>[5x]GMEVLDLVTGPDSVTEIEAFLNPRMGQPPTPESLTEGGQYYGWSRGINLATSDTEDSPENNTLPTWSMAKLQLPMLNEDLTCDTLQMWEAVSVKTEVVGSGSLLDVHGFNKPTDTVNTKGISTPVEGSQYHVFAVGGEPLDLQGLVTDARTKYKEEGVVTIKTITKKDMVNKDQVLNPISKAKLDKDGMYPVEIWHPDPAKNENTRYFGNYTGGTTTPPVLQFTNTLTTV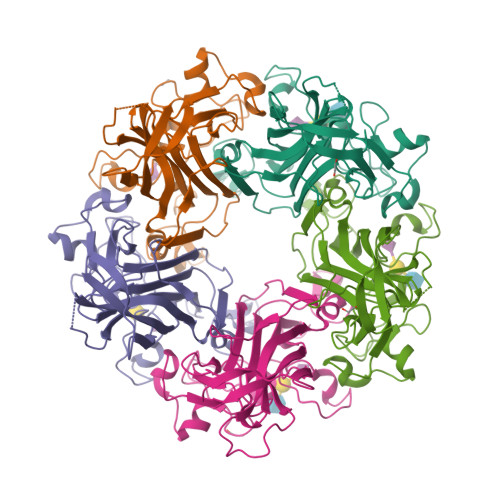LLDENGVGPLCKGEGLYLSCVDIMGWRVTRNYDVHHWRGLPRYFKITLRKRWVK>GPAMKRARSANIPGAILHSLAELQDGLNAMIDPSWRAVRSLDNWALAITMESTELLDSYPWKWWKNLNATP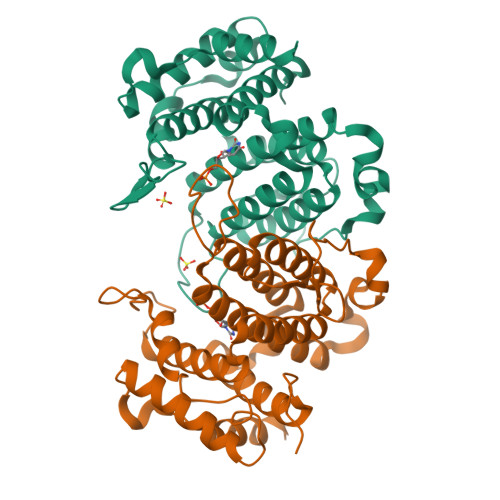DLANVRIELVDIFHFSLSGAMQMRSTPDDEIPAASLKPLKEVMTTFLPAKECTSDPYGFVFFPLTDTQNAIASFRNIIQLANAYRFDVIIECIIYAAEDLGFNLVAYYIAKHTLNCIRQLSGYKDGSYVKVNNGVEDNSLLHNCIKDVSLDEVLDADKYVQAWNSIMANVYEAFQIKESDRKDAERWFALAKENRLAIKA[4x]>AEAESALEYAQQALEKAQLALQA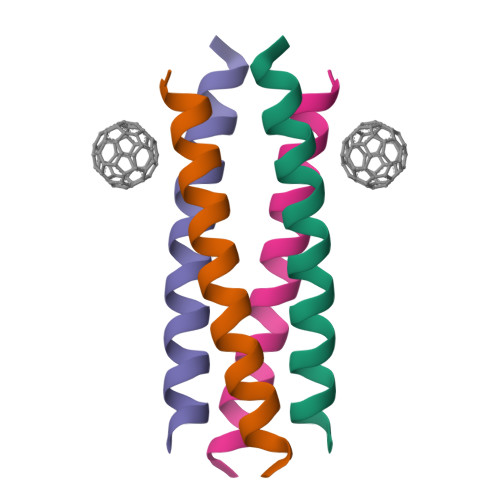ARQALKA[2x]>MSKKHTGYVGLKNQGATCYMNSLLQTLFFTNQLRKAVYMMPTEGDDSSKSVPLALQRVFYELQHSDKPVGTKKLTKSFGWETLDSFMQHDVQELCRVLLDNVENKMKGTCVEGTIPKLFRGKMVSYIQCKEVDYRSDRREDYYDIQLSIKGKKNIFESFVDYVAVEQLDGDNKYDAGEHGLQEAEKGVKFLTLPPVLHLQLMRFMYDPQTDQNIKINDRFEFPEQLPLDEFLQKTDPKDPANYILHAVLVHSGDNHGGHYVVYLNPKGDGKWCKFDDD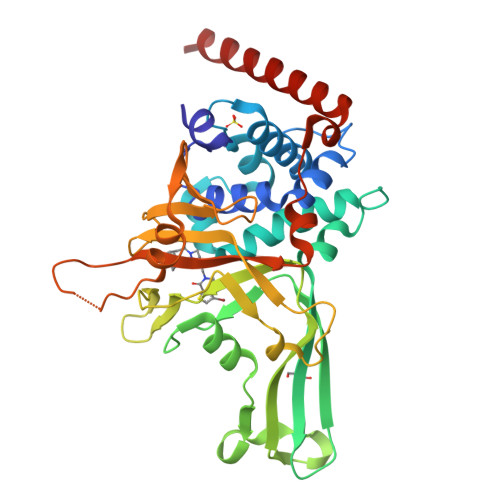VVSRCTKEEAIEHNYGGHDDDLSVRHCTNAYMLVYIRESKLSEVLQAVTDHDIPQQLVERLQEEKRIEAQKRKERQEHH[2x]>[2x]SMTYDKIKVPAQGEAITVAADHSLHVPDNPIIPFIEGDGIGVDVTPPMIRVVDAAVQKAYGNKRKISWMEVYAGEKATKVYGGDQWLPKETLDAMKKYVVSIKGPLTTPVGGGIRSLNVAIRQDMDLYVCLRPIRYFNGVPSPVREPWKTDMVIFRENSEDIYAGIEWQADTPEAKKVIQFLTKEMGVKKIRFPEHCGIGVKPVSREGTTRLVKAAIQY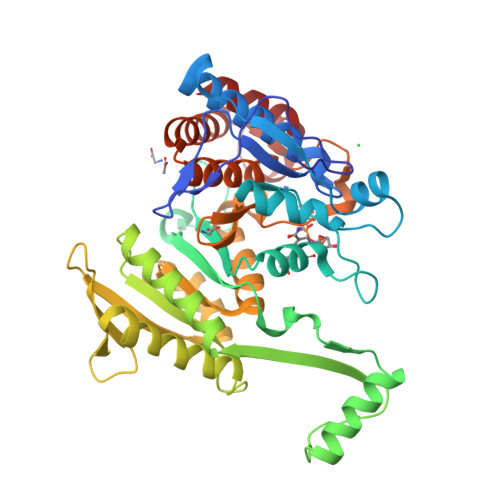AIDNDRSTVTLVHKGNIMKFTEGAFKDWGYQVARDSFGAKEYQGGPWMEFKNPKTGKQIIINDVIADAFLQQILLRPEDYSVIATLNLNGDYISDALAAQVGGIGIAPGANISDQMAVFEATHGTAPKYAGQNKVNPGSIILSAEMMLRHMGWYEAADLIIRGMEGAIEAKTVTYDFERGMQGATLVSSSGFADAMIKHM>NAMIIRPEQHWFLRLFDWHGSVLSKIIFRLLLNVLMSIIAIISYQWYEQLGIHLTVAPFSLLGIAIAIFLGFRNSASYSRFVEARNLWGTVLIAERTLVRQLRNILPAEHDAHRRIVSYLVAFSWSLKHQLRKTDPTADLRRLLPEERVTEILASSMPTNRILLLAGNEIGQLREAGKLSDITYGLMDNKLDELAHVLGGCERLATTPVPFAATLILQRTVYLFCTLLPFALVGDLHYMTPFVSVFISYTFLSWDSLAEELEDPFGTAANDLPLNAMCNTIERNLLDMTGQHPLPE[5x]

Human bestrophin1 (hBest1) is a Ca2+-activated Cl− channel essential for Cl− transport in retinal pigment epithelium (RPE). Although the structure of hBest1 is still unsolved, two Best1 homolog structures, one from bacteria Klebsiella pneumoniae (KpBest) and the other from chicken (cBest1), have been previously reported. Overall, the channel is a pentameric assembly with a single ion-conducting pathway, which varies in diameter along its length and is constrained at two narrow points: a “neck” contributed by three residues (I62/I66/F70 in KpBest and I76/F80/F84 in hBest1/cBest1) on a transmembrane helix, and an “aperture” formed by a single residue (I180 in KpBest1, I205 in hBest1, and V205 in cBest1) on a cytosolic helix. Here, by electrophysiological and structural analyses, we show that the neck and aperture in hBest1 are both indispensable Ca2+-dependent gates, and their dysregulated opening by rationally designed or patient-derived mutations causes Ca2+-independent leak and elevates Ca2+-dependent channel activity.

To further investigate Y236 and W287 on hBest1, we examined two mutants of each residue, including their individual alanine substitution mutants (Y236A and W287A), Y236C (a patient-derived mutation), and W287F (a milder alteration compared to W287A), all of which showed normal overall expression and membrane trafficking in HEK293 cells after transient transfection. The Y236A, Y236C, and W287F mutants all conducted Ca2+-dependent Cl− currents significantly bigger than those from WT hBest1 under the same conditions, indicating gain-of-function phenotypes. As the cBest1 3A mutant structure shows a constantly unconstrained neck, the gain-of-function in Y236A, Y236C, and W287F is likely a result of enhanced open probability of the neck. To understand the structural bases of these mutants, we solved the structures of KpBest Y211A, W252A, and W252F at 2.6, 2.5, and 3.1 Å (equivalent to hBest1 Y236A, W287A, and W287F), respectively. Consistent with the functional results, no structural change was found at the aperture. Although the structure at the neck region was surprisingly unaltered, possibly due to the molecular packing effect in the crystal or the presence of Zn2+ in the crystallization solution which might stabilize the channel in a closed state, all three KpBest mutants displayed conformational changes on P208, Y211, and W252 (equivalent to P233, Y236, and W287 in hBest1, respectively), reaffirming the mutual influence between these three residues. Taken together, we concluded that hBest1 P233, Y236, and W287 are critical residues involved in channel gating at the neck. Importantly, F80 and F84 are stabilized in the open conformation by interactions with hydrophobic residues Y236 and W287.2-[(S)-(2-chlorophenyl){2-[(2S)-1-methylpyrrolidin-2-yl]ethoxy}methyl]thieno[3,2-b]pyridine-7-carboxylic acid | C22 H23 Cl N2 O3 S | 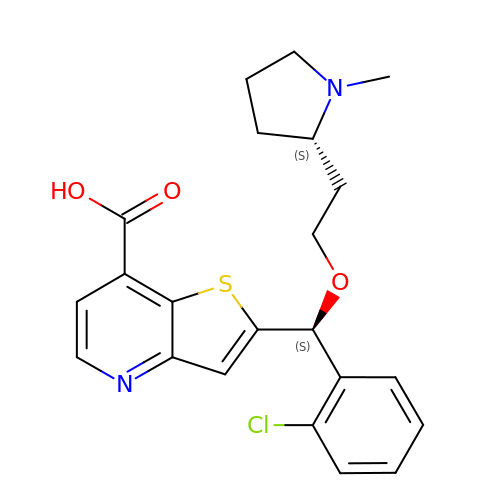CKHGFLIUOABPPV-XOBRGWDASA-N>[2x]MSLKQDLLNDRIILVTGASDGIGR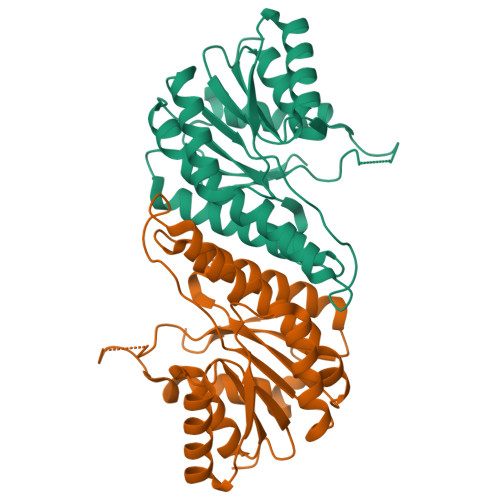EAAMTYARYGATVILLGRNEEKLRQVASHINEETGRQPQWFILDLLTCTSENCQQLAQRIVVNYPRLDGVLHNAGLLGDVCPMSEQNPQVWQDVMQINVNATFMLTQALLPLLLKSDAGSLVFTSSSVGRQGRANWGAYAASKFATEGMMQVLADEYQQRLRVNCINPGGTRTAMRASAFPTEDPQKLKTPADIMPLYLWLMGDDSRRKTGMTFDAQPGRKPGEGHHHHHH>GHMAESQALSDDIGFLLSRVGGMVLGAVNKALVPTGLRVRSYSVLVLACEQAEGVNQRGVAATMGLDPSQIVGLVDELEERGLVVRTLDPSDRRNKLIAATEEGRRLRDDAKARVDAAHGRYFEGIPDTVVNQM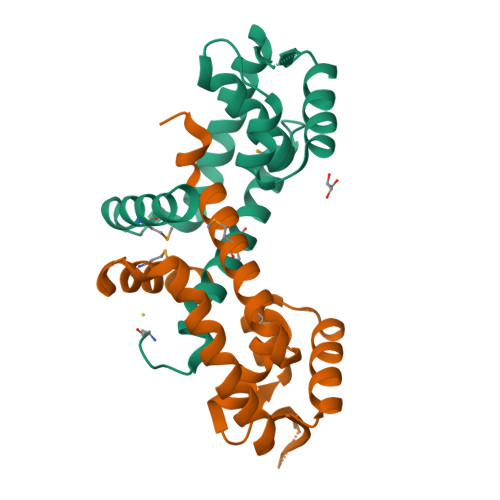RDTLQSIAFPTFVEGS[4x]>NVKKITKQLTLSLKNPFIYHHVVYGQNVLPGLAYIDIIYQIFREHGFSCSELQLRNLSIYQPLTAEQDAVI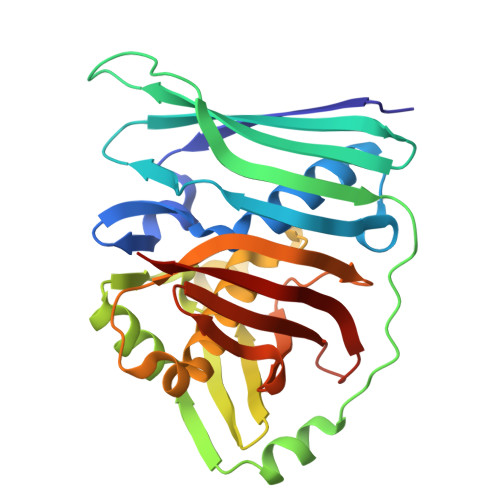VLNIQCAEKKEGQWQITAKGIEKRDGKEASEEKLYMKADMHADSPAIFEETLDLSQIKASAQNVVQLDDVYEQCRRQELVHSEYMKAKGCIYEEEDGVLLELSLGSEAMLHAEGFMFHPTLIDGSGVGANHLLTSLLKGEQRLYLPLFYESFSASALLQTDCMTRIKRSSVRREKELIYVTLEFFNASGEKVAELKNFTSKLV[2x]>AGGKVTSSTGIAPKRYVYYPGSEELGPDEIRVIACGTGMPTARRAQAAAAWVVELGNGDKFIVDIGSGSMANIQSLMIPANYLTKIFLTHLHTDHWGDLVSMWAGGWTAGRTDPLEVWGPSGSREDMGTKYAVEHMLKAYNWDYMTRAVTINPRPGDINVHEFDYRALNEVVYQENGVTFRSWPCIHAGDGPVSFALEWNGYKVVFGGDTAPNIWYPEYAKGADLAIHECWMTSDQMMTKYNQPAQLALRINLDFHTSAQSFGQIMNMVQPRHAVAY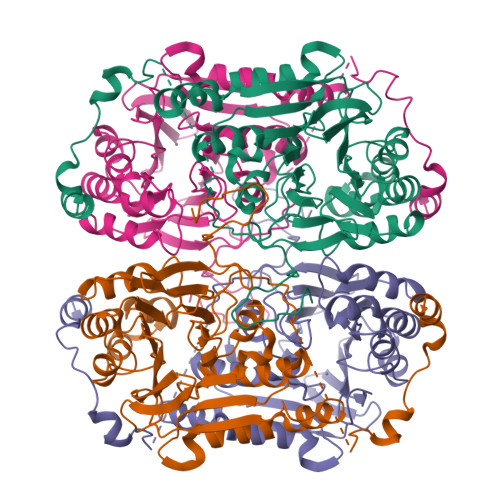AFFNDDDTRYDIYTGVRENYAGPLSMATDMMVWNITRDAVTERMAVSPDHAWDVAGPSEDLAPDRNRASEYTQYILDGRLNVDEANAHWKQEFMG[4x]> KGTFKDYVRDRADLNKDKPVIPAAALAGYTG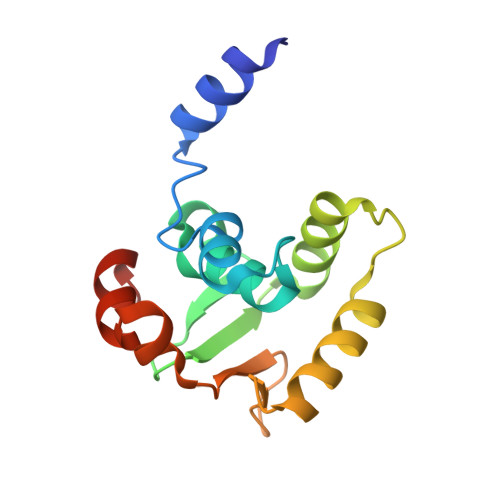SGPIQLWQFLLELLTDKSCQSFISWTGDGWEFKLSDPDEVARRWGKRKNKPKMNYEKLSRGLRYYYDKNIIHKTAGKRYVYRFVCDLQSLLGYTPEELHAMLDVKPDAD>[10x]VPRGSQNFLFGCELKADKKEY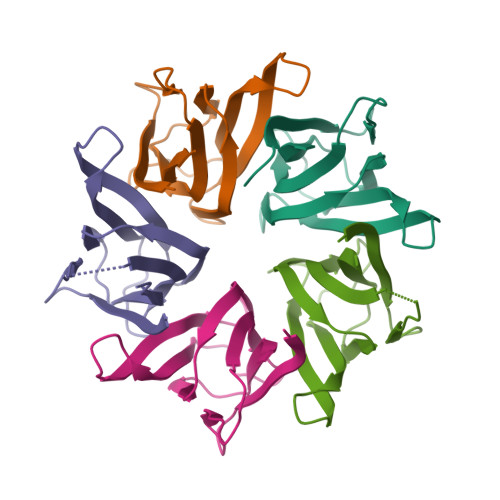SFKVEDDENEHQLSLRTVSLGASAKDELHVVEAEGINYEGKTIKIALASLKPSVQPTVSLGGFEITPPVILRLKSGSGPVYVSGQHLVALEDL>PEVAVTGQVLETLPPIGVFWDIENCSVPSGRSATTVVQRIREKFFRGHREAEFICVCDISKENKEVIQELNNCQVTVA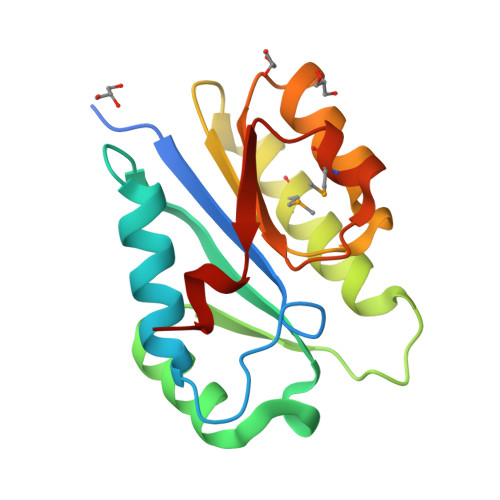HINATAKNAADDKLRQSMRRFANTHTAPATVVLVSTDVNFALELSDLRHRHGFHIILVHKNQASEALMHHANQLIRFEEFISDLP[4x]> STIPGSAATLNTSITKNIQNGNAYIDLYDVKLGKIDPLQLIVLEQGFTAKYVFRQGTKYYGDVSQLQSTGRASLTYNIFGEDGLPH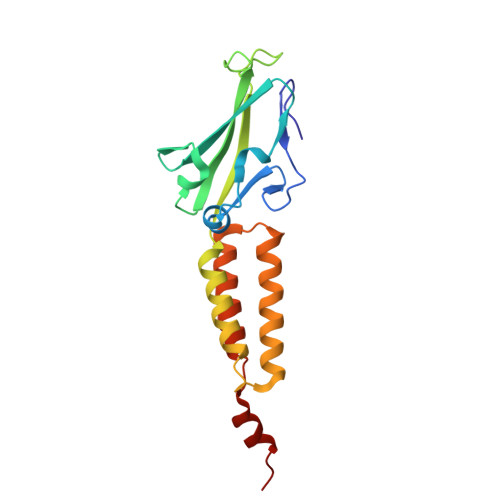VKTDGQIDIVSVALTIYDSTTLRDKIEEVRTNANDPKWTEESATEVLTGLDTIKTDIDNNPKTQTDIDSKIVEVNELEKLLVLKLAAALEHHHH6-methyl-5,6,6~{a},7-tetrahydro-4~{H}-dibenzo[de,g]quinoline-10,11-diol | C17 H17 N O2 | 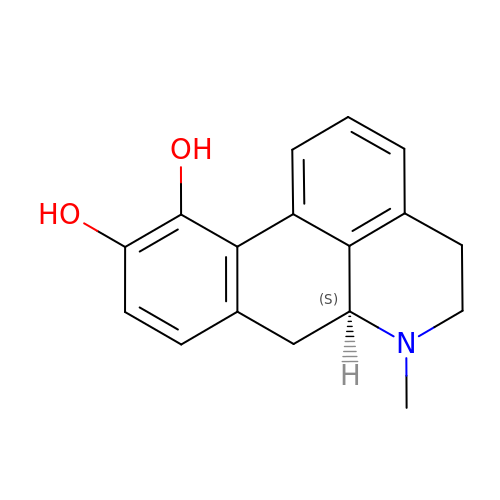VMWNQDUVQKEIOC-ZDUSSCGKSA-N> MAETKSMFREVLPKQGQLYVEDITTMVLCKPKLLPLKSLTLEKLEKMQQAAQDTIHQQEMTEKEQKITH;> MAATSSSDSDGGKGESEANSKWLDSLSDSMANIHTFSACLALADFHGDGEYKLAMGDLGPDGRQPRLKVLKGHTLVSQKPLPDLPAAAVTFLMASHEPRTPALAIASGPCVYVYKNLKPYFKFSLPSLPTNPLEQDLWNQAKEDQIDPLTLKEMLEGIREKAEVPLSVQSLRFLPLELSEMEAFVNQHKSKSIRRQTVITTMTTLKKNLADEDAVSCLVLGTENKELLVLDPEAFTILAKMSLPSVPAFLEASGQFDVEFRLAAACRNGSIYILRRDSKRPKYCIELGAQPVGLVGVHKVLVVGSNQDSLHGFTYKGKRLWTVQMPAAILAMNLLEQHSRGLQAVMAALANEEVRIYHDKVLLNVIRTPEAVTSLCFGRYGREDNTLIMTTLGGGLIIKILKRTAVFAEGGGEAGPPPSQAIKLNVPRKTRLYVDQTLREREAGTAMHRTFQADLYLLRLRAARAYVQALESSLSPVSLTAREPLKLHAVVQGLGPTFKLTLHLQNTSTARPILGLVVCFLYNEVLYALPRAFFKVPLLVPGLNYPLETFVKSLSDKGISDIIKVLVLREGQSTPLLSAHINMPMSEGLAAD;> MLQPVFTLKLRHKISPRMVAVGRYDGTHPCLAAATQAGKVFIHNPHSRSQHLGAPRVLQSPLESDVSLLNINQTVSCLTAGVLNPELGYDALLVGTQTNLLAYDVYNNSDLFYREVADGASAIVLGTLGDITSPLAIIGGNCALQGFNHEGNDLFWTVTGDNVHSLALCDFDGDGKKELLVGSEDFDIRVFKEDEIVAEMSETEIITSLCPMYGSRFGYALSNGTVGVYDKTARYWRIKSKNQAMSIHAFDLNSDGVCELITGWSNGKVDARSDRTGEVIFKDNFSSAIAGVVEGDYRMEGCQQLICCSVDGEIRGYLPGTAEMRGNLMDISVEQDLIRELSQKKQNLLLELRNYEENAKAELSSPLNEADGHRGVIPANTKHHTALSVSLGSEAQAAHAELCISTSNDTIIRAVLIFAEGVFAGESHVVHPSVHHLSSSVRIPITPPKDIPVDLHLKTFVGYRSSTQFHVFELTRQLPRFSMYALTSPDPASEPLSYVNFIIAERAQRVVMWLNQNFLLPEDTNIQNAPFQVCFTSLRNGGQLYIKIKLSGEITVNTDDIDLAGDIIQSMASFFAIEDLQVEADFPVYFEELRKVLVKVDEYHSVHQKLSADMADNSNLIRSLLVQAEDARLMRDMKTMKNRYKELYDLNKDLLNGYKIRCNNHTELLGSLKAVNQAIQRAGHLRVGKPKNQVITACRDAIRSNNINMLFRIMRVGTASS;> MGLLDRLSGLLGLKKKEVHVLCLGLDNSGKTTIINKLKPSNAQSQDIVPTIGFSIQKFKSSSLSFTVFDMSGQGRYRNLWEHYYKEGQAIIFVIDSSDKLRMVVAKEELRTLLNHPDIKHRRIPILFFANKMDLRDALTSVKVSQLLCLEDIKDKPWHICASDAIKGEGLQEGVDWLQDQIQSVKT;> MAEEKLSARTQLPVSAESQKPVLKKAPEFPILEKQNWLIHLYYIQKDYEACKAVIKEQLQETHGLCEYAIYVQALIFRLEGNIQESLRLFQMCAFLSPQCADNLKQVARSLFLLGKHKAAIEVYNEAAKLNQKDWEICHNLGVCYIYLKQFDKAQDQLHNALHLNRHDLTYIMLGKIFLLKGDLDKAIEIYKKAVEFSPENTELLTTLGLLYLQLGIYQKAFEHLGNTLTYDPTNYKAILAAGSMMQTHGDFDVALTKYKVVACAVIESPPLWNNIGMCFFGKKKYVAAISCLKRANYLAPLDWKILYNLGLVHLTMQQYASAFHFLSAAI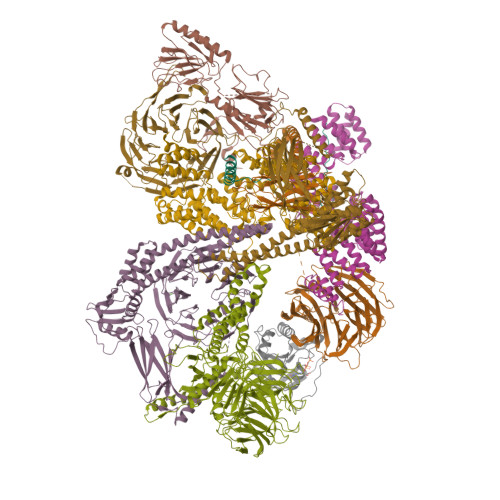NFQPKMGELYMLLAVALTNLEDSENAKRAYEEAVRLDKCNPLVNLNYAVLLYNQGEKRDALAQYQEMEKKVNLLKYSSSLEFDPEMVEVAQKLGAALQVGEALVWTKPVKDPKSKHQTASTSKAAGFQQPLGSNQALGQAMSSAATCRKLSSGAGGTSQLTKPPSLPLEPEPTVEAQPTEASAQTREK;> MSVLDALWEDRDVRFDVSSQQMKTRPGEVLIDCLDSVEDTKGNNGDRGRLLVTNLRIVWHSLALPRVNLSIGYNCILNITTRTANSKLRGQTEALYVLTKCNSTRFEFIFTNLVPGSPRLYTSLIAVHRAYETSKMYRDFKLRSALIQNKQLRLLPQENVYNKINGVWNLSSDQGNLGTFFITNVRIVWHANMNDSFNVSIPYLQIRSVKIRDSKFGLALVIESSQQSGGYVLGFKIDPVEKLQESVKEINSLHKVYSANPIFGVDYEMEEKPQPLEALTVKQIQDDVEIDSDDHTDAFVAYFADGNKQQDREPVFSEELGLAIEKLKDGFTLQGLWEVMN;> MDLNLNRADYLQVGVTSQKTMKLLPASKHRATQKVVVGDHDGIVMCFGMKKGEAVTVFKTLPGQKIARLELGGALNTPQEKIFIAAGSEIRGFTKRGKQFLSFETNLTESIKAMHISGSDLFLSASYIYNHYCDCKDQHYYLSGDKINDVICLPVERLLREVPVLACQDRVLRVLQGSDVTYEIEVPGPPTVLALHNGNGGDSGEDLLFGTSDGKLGLIQITTSKPIHKWEIRNEKKRGGILCVDSFDIVGDGVKDLLVGRDDGMVEVYGFDNANEPVLRFDHTLSESVTSIQGGCVGKDGYDEIVVSTYSGWITGLTTEPVHKESGPGEELKFNQEMQNKISSLRSELEQLQYKVLQEREKYQQSSQSSKAKSAVPSFSVNDKFTLNKDDASYSLILEVQTAIDNVLIQSDVPIDLLDVDKNSAVVSFSSCDSESNDNFLLATYRCQANTTRLELKIRSIEGQYGTLQAYVTPRIQPKTCQVRQYHIKPLSLHQRTHFIDHDRPMNTLTLTGQFSFSELHSWVVFCMPEVPEKPPAGECVTFYFQNTFLDTQLESTYRKGEGVFKSDNISTISILKDVLSKEATKRKINLNISYEINEVSVKHTLKLIHPKLEYQLLLAKKVQLIDALKELQVHEGNTNFLIPEYRCILEEADHLQEEYKKQPAHLERLYGMITDLFIDKFKFKGTNVKTKVPLLLEILDSYDQNALIAFFDAA;> MEPLLLAWSYFRRRRFQLCADLCTQMLEKSPCDQAAWILKARALTEMVYVDEIDVDEEGIAEMILDENAIAQVPRPGTSLKLPGTNQTGGPSPAVRPVTQAGRPITGFLRPSTQSGRPGTIEQAIKTPRTAYTARPIASSSGRFVRLGTASMLTSPDGPFINLSRLNLAKYAQKPKLAKALFEYIFHHENDVKTALDLAALSTEHSQYKDWWWKVQIGKCYYRLGLYREAEKQFKSALKQQEMVDTFLYLAKVYISLDQPLTALNLFKQGLDKFPGEVTLLCGIARIYEEMNNISSATEYYKEVLKQDNTHVEAIACIGSNHFYTDQPEVALRFYRRLLQMGVYNCQLFNNLGLCCFYAQQYDMTLTSFERALSLAENEEEVADVWYNLGHVAVGTGDTNLAHQCFRLALVSNNQHAEAYNNLAVLEMRRGHVEQAKALLQTASSLAPHMYEPHFNFATISDKIGDLQRSYAAAKKSEAAFPDHVDTQHLIKQLEQHFAML;> MSLFKARDWWSTVLGDKEEFDQGCLCLADVDNTGNGQDKIIVGSFMGYLRIFNPHPVKTGDGAQAEDLLLEVHLRDPILQVEVGKFVSGTEMLHLAVLHSRKLCVYSVSGTLGNVEHGNQYQIKLMYEHNLQRTACNMTYGSFGGVKGRDLICIQSVDGMLMVFEQESYAFGRFLPGSLLPGPLAYSSRTDSFITVSSCHQVESYKYQVLAFATDADKRQETEQQKHGSGKRLVVDWTLNIGEQAIDICIVSFIQSASSVFVLGERNFFCLKDNGQIQFMKKLDYSPSCFLPYCSVSEGTINTLIGNHNNMLHIYQDVTLKWATQLPHVPVAVRVGCLHDLKGVIVTLSDDGHLQCSYLGTDPSLFQAPKVESRELNYDELDMELKELQKVIKNVNKSQDVWPLTEREDDLKVSAMVSPNFDSVSQATDVEVGADLVPSVTVKVTLKNRVALQKIKLSIYVQPPLVLTGDQFTFEFMAPEMTRTVGFSVYLKGSYSPPELEGNAVVSYSRPTERNPDGIPRVSQCKFRLPLKLVCLPGQPSKTASHKLTIDTNKSPVSLLSLFPGFAKQSEDDQVNVMGFRFLGGSQVTLLASKTSQRYRIQSEQFEDLWLITNELIIRLQEYFEKQGIKDFTCSFSGSVPLEEYFELIDHHFELRINGEKLEELLSERAVQFRAIQRRLLTRFKDKTPAPLQHLDTLLDGTYKQVIALADAVEENQDNLFQSFTRLKSATHLVILLIGLWQKLSADQIAILEAAFLPLQQDTQELGWEETVDAALSHLLKTCLSKSSKEQALNLNSQLGIPKDTSQLKKHITLFCDRLAKGGRLCLSTDAAAPQTMVMPGGCATIPESDLEGRSIDQDSSELFTNHKHLMVETPVPEVSPLQGVTE>GAMGSPGDGAGASRQRKLEALIRDPRSPINVESLLDGLNSLVLDLDFPALRKNKNIDNFLNRYEKIVKKIRGLQMKAEDYDVVKVIGRGAFGEVQLVRHKAS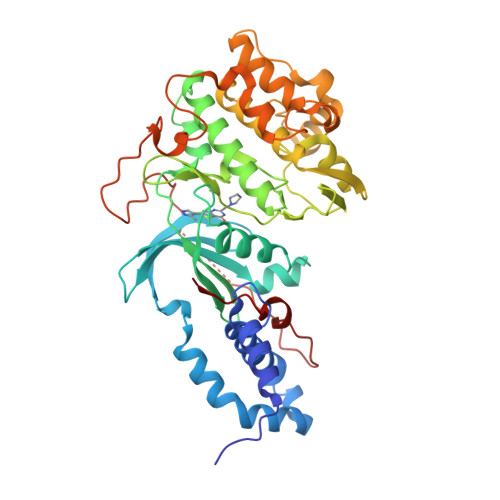QKVYAMKLLSKFEMIKRSDSAFFWEERDIMAFANSPWVVQLFYAFQDDRYLYMVMEYMPGGDLVNLMSNYDVPEKWAKFYTAEVVLALDAIHSMGLIHRDVKPDNMLLDKHGHLKLADFGTCMKMDETGMVHCDTAVGTPDYISPEVLKSQGGDGYYGRECDWWSVGVFLYEMLVGDTPFYADSLVGTYSKIMDHKNSLCFPEDAEISKHAKNLICAFLTDREVRLGRNGVEEIRQHPFFKNDQWHWDNIRETAAPVVPELSSDIDSSNFDDIEDDKGDVETFPIPKAFVGNQLPFIGFTYYR[4x]>MELYLDTSDVVAVKALSRIFPLAGVTTNPSIIAAGKKPLDVVLPQLHEAMGGQGRLFAEVMATTAEGMVNDALKLRSIIADIVVKVPVTAEGLAAIKMLKAEGIP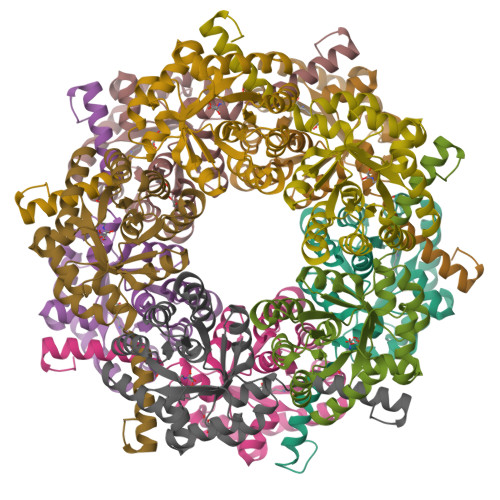TLGTAVYGAAQGLLSALAGAEYVAPYVNRIDAQGGSGIQTVTDLHQLLKMHAPQAKVLAASFKTPRQALDCLLAGCESITLPLDVAQQMISYPAVDAAVAKFEQDWQGAFGRTSI[10x]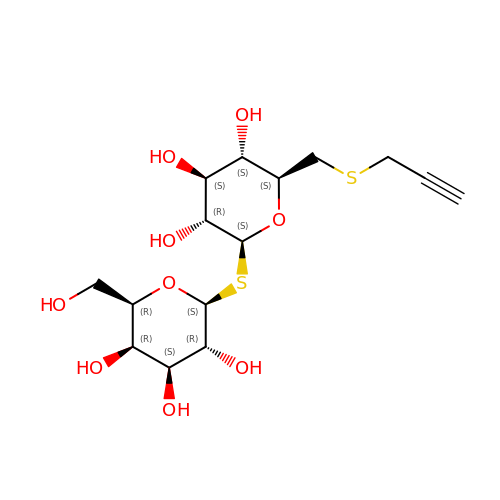6-S-(prop-2-yn-1-yl)-6-thio-beta-D-glucopyranosyl 1-thio-beta-D-galactopyranoside | C15 H24 O9 S2 | VMLLJSJIKUKSIE-PHOFNFIUSA-N> GAMTFTRYSRLRVIAEIRHGDIFHSANIVSSIEFDRDDELFATAGVSRCIKVFDFSSVVNEPADMQCPIVEMSTRSKLSCLSWNKHEKNHIASSDYEGIVTVWDVTTRQSLMEYEEHEKRAWSVDFSRTEPSMLVSGSDDCKVKVWCTRQEASVINIDMKANICCVKYNPGSSNYIAVGSADHHIHYYDLRNISQPLHVFSGHKKAVSYVKFLSNNELASASTDSTLRLWDVKDNLPVRTFRGHTNEKNFVGLTVNSEYLACGSETNEVYVYHKEITRPVTSHRFGSPDMDDAEEEAGSYFISAVCWKSDSPTMLTANSQGTIKVLVLAA;> XYLQIVPEIHK

The COP1 E3 ubiquitin ligase is a central signaling hub that integrates inputs from plant light‐sensing photoreceptors. COP1 contains an N‐terminal zinc finger, a central coiled‐coil, and a C‐terminal WD40 domain, which is essential for proper COP1 function (Deng et al, 1992; McNellis et al, 1994). COP1 regulates gene expression and plays a central role as a repressor of photomorphogenesis by directly modulating the stability of transcription factors that control the expression of light‐regulated genes.

We mapped putative VP motifs in all these proteins and assessed their binding affinities to the COP1 WD40 domain. We could detect binding for most of the peptide motifs in ITC assays, with dissociation constants in the mid‐micromolar range (Figs 4A and EV4). Next, we obtained crystal structures for the different peptides bound to COP1 (1.3–2.0 Å resolution, see Tables EV1 and EV2, and EV4) to compare their peptide binding modes. We found that all peptides bind in a similar configuration with the VP forming the center of the binding site (r.m.s.d. between the different peptides range from ~ 0.3 to 1.5 Å, comparing 5 or 6 corresponding Cα atoms). In yeast 3‐hybrid assays, we find that, similar to HY5, UV‐B‐activated UVR8 can efficiently compete with HYH and an N‐terminal fragment of HFR1 for binding to COP1 (Fig EV5).> GAACGACATTGA;> CGACGACTC;> TCATCG;> TCGAGTCAGTGTCGT

In this work, we exhaustively probe the ability of all 36 immobile HJ sequences to form DNA crystals in two different designed systems. Three separate self-assembling DNA crystal systems are described in this report: the “4 × 5” and “4 × 6” designs (collectively referred to as the 4 × N systems), and a third construct with a “scrambled” sequence variant of the 4 × 6 lattices. Self-assembly was mediated by three constituent oligonucleotides: (S1) containing four sequence repeats of either 5 or 6 bases; (S2) composed of 21 bases containing complementary regions to both (S1); and (S3) which forms the second junction crossover. The HJ serves as the fundamental component at the core of each unit, and the ultimate assembly of the full lattice is facilitated by the complementary 2-base sticky ends that tail each duplex.

To investigate this possibility, we designed “scrambled” sequences with targeted base substitutions, while maintaining GC content, along each “stem”. Contrary to the buffer preference observed with the native P32 crystals, the scrambled systems exhibited an exclusive preference towards low salt buffers, much like the native R3 crystals. Remarkably, only J1 and J2 retained the P32 symmetry, with all others yielding an R3 lattice. There appeared to be only a marginal difference in the average cell lengths in the R3 scramble crystals (a = b = 113.04 c = 51.10) relative to the native 4 × 6 sequences: the a, b axis trended ~2 Å shorter and c ~1.3 Å longer, whereas in the J1 and J2 cases, the crystals were in good agreement with the original 4 × 6 motif. The average angles of the R3 and P32 crystals were 61.00° (σ = 1.21) and 58.05° (σ = 1.39), respectively. Another major observation is the importance of stem region sequences outside the HJ, given that this sequence can control crystal symmetry and lattice architecture, and improve resolution in non-obvious ways. However, in the majority of the crystal structures reported here, the cacodylate anion indeed fits best into the electron density map of our X-ray structures, due to the presence of sodium cacodylate in the crystallization solution.>SNAMTKVAIVTASDSGIGKTTALMLAERGFDIGVTWHSDEQGARDTCREVEAQGRRAEAIHLDLSTLPQGAQAIETLIARFGRLDVLVNNAGAMTKAPFLDMPFDDWRNIFTVDVDGAFLCSQIAARKMVEQGEGGRIVNITSVHEHTPLPEASAYTAAKHALGGLTKSMALELVQHNILVNAVAPGAIATPMNDMDESEVKEGSMPAIPLARPGYTKE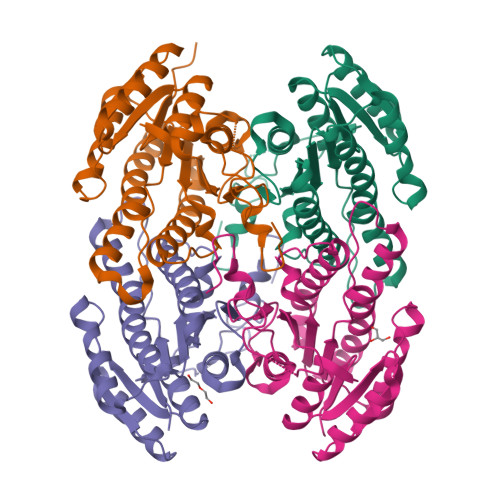IASLVAWLCDSDASYTTGQSFIVDGGFMLANPQFKPEG[4x]> PFLELDTNLPANRVPAGLEKRLCAAAASILGKPADRVNVTVRPGLAMALSGSTEPCAQLSISSIGVVGTAEDNRSHSAHFFEFLTKELALGQDRILIRFAPLESWQIGKIGTVMTFL

pmcThe human macrophage migration inhibitory factor (MIF) superfamily, comprised of MIF and D-dopachrome tautomerase (DDT, also called MIF-2), is broadly and constitutively expressed with involvement in proinflammatory and host antimicrobial responses. MIF and MIF-2 are highly similar in structure, with monomeric units of 114 and 117 amino acids, respectively, that form homotrimers. An evolutionarily conserved proline at the N terminus acts as the catalytic base for a tautomerization reaction of unknown biological significance in both proteins. The same site in MIF-2 is Phe100 and is also evolutionarily conserved among all MIF-2 proteins, suggesting this site plays an important role in both proteins.

In agreement with MIF enzyme kinetics, the activity was decreased in the S62A and F100A variants by 13% and 60% (versus wt-MIF-2), respectively. The substantial change in F100A enzymatic activity despite ∼9 Å between the mutation and catalytic sites implies long-range communication within the MIF-2 structure. Surprisingly, the F100A variant has a higher RMSD (1.245 Å) with wt-MIF-2, displaying substantial conformational changes in the β-strand housing the F100A mutation, the C-terminal region, and the loop 63 to 69 connecting the third β-strand to the second α-helix. These changes were not observed in the Y99A MIF mutant, but in MIF-2, this mutation induces the adjacent Pro101 from each subunit to form a “lid” over the solvent cavity to separate external and internal water molecules. There are significant differences in the F100A variant including a conformational change in the active site residue Ile64 and increased dynamics of the active site Arg36 and C-terminal Met114 side chains (dynamics are interpreted from the absence of electron density). In addition, the expansion in the F100A variant is also only 0.9 Å due to the loss of the large side chain near the mouth of the cavity and movement of Pro101 into this space, a conformational change not observed in Tyr99 MIF variants. There is an even slightly smaller network of water molecules trapped between Pro101 and Arg42 in F100A MIF-2, which has a kcat/Km ∼40% of wt-MIF-2. It must be noted that changes in the F100A water network are partly due to the truncation of the solvent cavity from multiple conformational changes. However, F100A displays more line broadening, particularly in residues 60 to 65 that were noted to undergo a conformational change in the F100A crystal structure. The P1G and F100A variants show similar levels of dynamic perturbation; however, the effects of F100A are strongest at the C terminus, most notably residues Ile107 and Ile110, which have been purported to be involved in CD74 activation. Before our X-ray structure of F100A MIF-2 showed significant conformational changes, it was unclear why a Phe100 mutation would have a larger effect on the activity in MIF-2.>[2x]MFGIFDKGQKIKGTVVLMPKNVLDFNAITSIGKGGVIDTATGILGQGVSLVGGVIDTATSFLGRNISMQLISATQTDGSGNGKVGKEVYLEKHLPTLPTLGARQDAFSIFFEWDASFGIPGAFYIKNFMTDEFFLVSVKLEDIPNHGTIEFVCNSWVYNFRSYKKNRIFFVNDTYLPSATPAPLLKYRKEEFEVLRGDGTGKRKDFDRIYDYDVYNDLGNPDGGDPRPILGGCSIYPYPLRVRTGRERTRTDPNSEKPGEVYVPRDENFGHLKSSDFLTYGIKSLSHDVIPLFKSAIFQLRVTSSEFESFEDVRSLYEGGIKLPTDILSQISPLPALKEIFRTDGENVLQFPPPHVAKVSKSGVMTDEEFAR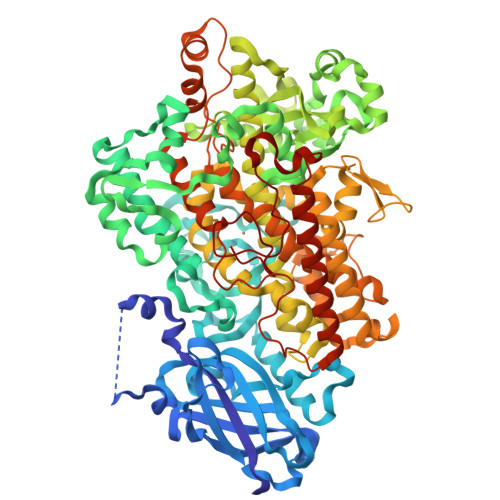EVIAGVNPNVIRRLQEFPPKSTLDPTLYGDQTSTITKEQLEINMGGVTVEEALSTQRLFILDYQDAFIPYLTRINSLPTAKAYATRTILFLKDDGTLKPLAIELSKPHPDGDNLGPESIVVLPATEGVDSTIWLLAKAHVIVNDSGYHQLVSHWLNTHAVMEPFAIATNRHLSVLHPIYKLLYPHYRDTININGLARQSLINADGIIEKSFLPGKYSIEMSSSVYKNWVFTHQALPADLVKRGLAIEDPSAPHGLRLVIEDYPYAVDGLEIWDAIKTWVHEYVSLYYPTDAAVQQDTELQAWWKEAVEKGHGDLKEKPWWPKKQTTEDLIQSCSIIVWTASALHAAVNFGQYPYGGLILNRPTLARRFIPAEGTPEYDEMVKNPQKAYLRTITPKFETLIDLSVIEILSRHASDEIYLGERETPNWTTDKKALEAFKRFGSKLTGIEGKINARNSDPSLRNRTGPVQLPYTLLHRSSEEGLTFKGIPNSISI>MAEQLVEAPAYARTLDRAVEYLLSCQKDEGYWWGPLLSNVTMEAEYVLLCHILDRVDRDRMEKIRRYLLHEQREDGTWALYPGGPPDLDTTIEAYVALKYIGMSRDEEPMQKALRFIQSQGGIESSRVFTRMWLALVGEYPWEKVPMVPPEIMFLGKRMPLNIYEFGSWARATVVALSIVMSRQPVFPLPERARVPELYETDVPPRRRGAKGGGGWIFDALDRALHGYQKLSVHPFRRAAEIRALDWLLERQAGDGSWGGIQPPWFYALIALKILDMTQHPAFIKGWEGLELYGVELDYGGWMFQASISPVWDTGLAVLALRAAGLPADHDRLVKAGEWLLDRQITVPGDWAVKRPNLKPGGFAFQFDNVYYPDVDDTAVVVWALNTLRLPDERRRRDAMTKGFRWIVGMQSSNGGWGAYDVDNTSDLPNHIPFCDFGEVTDPPSEDVTAHVLECFGSFGYDDAWKVIRRAVEYLKREQKPDGSWFGRWGVNYLYGTGAVVSA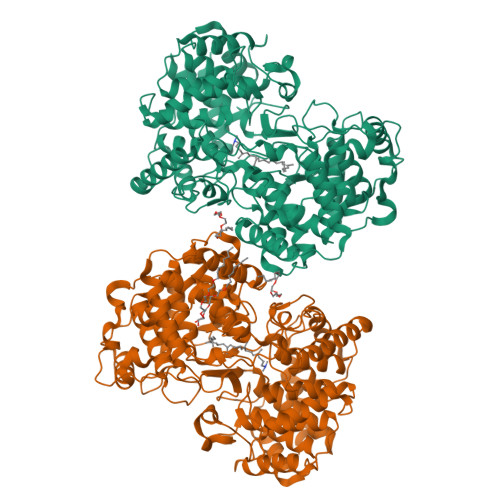LKAVGIDTREPYIQKALDWVEQHQNPDGGWGEDCRSYEDPAYAGKGASTPSQTAWALMALIAGGRAESEAARRGVQYLVETQRPDGGWDEPYYTGTGFPGDFYLGYTMYRHVFPTLALGRYKQAIERR[3x]>GENSDNLTHCRLFEFRLCLLECMSLTLDHCYARCTTVITQIHGSDTNRFDCTIFKTCYYRCYVLGKTEDHCW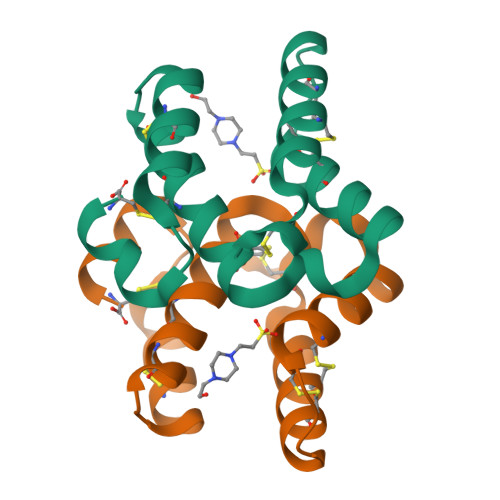KGTATSVTGDVGDLEFC[6x]>[2x]GSMASLPVLQKESVFQSGAHAYRIPALLYLPGQQSLLAFAEQRASKKDEHAELIVLRRGDYDAPTHQVQWQAQEVVAQARLDGHRSMNPCPLYDAQTGTLFLFFIAIPGQVTEQQQLQTRANVTRLCQVTSTDHGRTWSSPRDLTDAAIGPAYREWSTFAVGPGHCLQLNDRARSLVVPAYAYRKLHPIQRPIPSAFCFLSHDHGRTWARGHFVAQDTLECQVAEVETGEQRVVTLNARSHLRARVQAQS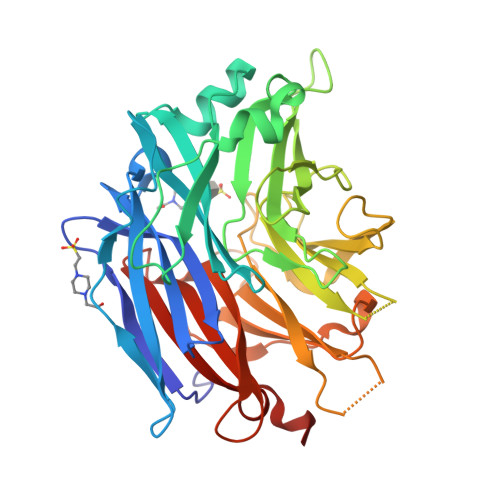TNDGLDFQESQLVKKLVEPPPQGCQGSVISFPSPRSGPGSPAQWLLYTHPTHSWQRADLGAYLNPRPPAPEAWSEPVLLAKGSCAYSDLQSMGTGPDGSPLFGCLYEANDYEEIVFLMFTLKQAFPAEYLPQ> CAAAGAAAAG;> CTXTCTTTG

With this in mind we describe reduced-charge oligonucleotides containing artificial LNA-amide linkages with improved gymnotic cell uptake, RNA affinity, stability and potency. We solved several X-ray structures to determine the effects of LNA and amide modifications on duplex structure and conformation. These are the first crystal structures of DNA:RNA hybrids that contain amide linkages. The sequence of the modified DNA:RNA hybrid duplexes was based on the corresponding unmodified version (d-CTTTTCTTTG/rCAAAGAAAAG)51 (the location of the amide is underlined).

Good quality crystals diffracting between 2.5–2.8 Å resolution were obtained for the DNA:RNA hybrid in which the DNA strand contains an amide linkage flanked by DNA on both sides, LNA on both sides and with LNA only on the 5′-side. The hybrids with amide and LNA-amide backbones are structurally very similar to the unmodified duplex (all-atom RMSD 0.4 Å) as shown by their superimposition. All structures adopt the A-conformation with sugar puckers clustering around C3′-endo. In agreement with the DNA:RNA hybrid NMR structure by Rosners22 in which the DNA strand contained multiple amides, our X-ray studies indicate that the amide linkage is a close mimic of the phosphodiester backbone. Both are four-atom linkages, hence similar in length, and the amide carbonyl is orientated in the same direction as one of the phosphodiester P-O bonds. Between each structure, the orientation of the backbone is consistent, directing the amide oxygen into the major groove. The amide adopts the expected trans-conformation, and LNA on the 5′-side of the amide has little effect on backbone torsion angles. In duplexes with DNA targets, ONs with all combinations of LNA and DNA sugars around the amide linkage were slightly destabilising (between −0.1 to −2.6 ˚C), indicating the selectivity of the amide linkage for complementary RNA.>[2x]AKKEIPLKYGATNEGKRQDPAMQKFRDNRLGAFIHWGLYAIPGGEWNGKVYGGAAEWLKSWAKVPADEWLKLMDQWNPTKFDAKKWAKMAKEMGTKYVKITTKHHEGFCLWPSKYTKYTVANTP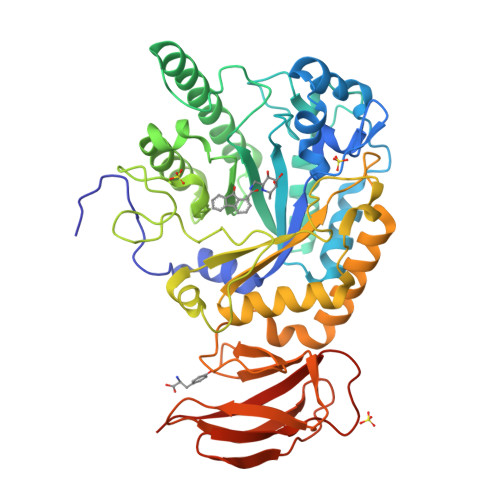YKRDILGELVKAYNDEGIDVHFYFSVMDWSNPDYRYDIKSKEDSIAFSRFLEFTDNQLKELATRYPTVKDFWFDGTWDASVKKNGWWTAHAEQMLKELVPGVAINSRLRADDKGKRHFDSNGRLMGDYESGYERRLPDPVKDLKVTQWDWEACMTIPENQWGYHKDWSLSYVKTPIEVIDRIVHAVSMGGNMVVNFGPQADGDFRPEEKAMATAIGKWMNRYGKAVYACDYAGFEKQDWGYYTRGKNDEVYMVVFNQPYSERLIVKTPKGITVEKATLLTTGEDITVVETTRNEYNVSVPKKNPGEPYVIQLKVRAAKGTKSIYRDALT>[2x]GAMESLPVIAAPSMWTRPQIKDFKEKIQQDADSVITVGRGEVVTVRVPTHEEGSYLFWEFATDNYDIGFGVYFEWTDSPNTAVSVHVSESSDDDEEEEENIGCEEKAKKNANKPLLDEIVPVYRRDCHEEVYAGSHQYPGRGVYLLKFDNSYSLWRSKSVYYRVYYTR;>[2x]GSGSGKPAPDAIGDLLASVDSEEVRQYCREQGWIIPETPTNVERHLNR

ACBD3 is a Golgi resident protein involved in the maintenance of the Golgi structure and regulation of intracellular trafficking between the endoplasmic reticulum and the Golgi. However, in enterovirus-infected cells, the ACBD3 GOLD domain interacts preferentially with viral non-structural 3A proteins, which causes re-localization of ACBD3 to the sites of virus replication. In this study, we present a structural, biochemical, and biological characterization of the complexes composed of human ACBD3 and the 3A proteins of four representative enteroviruses. The crystal structures revealed the details of the ACBD3-3A interaction, the 3A-3A interaction causing the assembly of the ACBD3-3A heterotetramers, the interaction between the ACBD3-3A complex and the lipid bilayer, and the roles of these interactions in facilitation of enterovirus replication.

The second strategy took advantage of the fact that in all three solved GOLD: 3A structures the C terminus of the ACBD3 GOLD domain was located in the vicinity of the N terminus of the ordered part of the 3A protein. This allowed us to design GOLD-3A fusion proteins with the last residue of ACBD3 (R528ACBD3) fused through a short peptide linker (GSGSG) to the first predicted ordered residues of the respective 3A proteins (e.g. K153A/EVA71). The overall structures of all solved GOLD: 3A complexes are highly similar to each other. This suggests that neither the L24A mutation in the GOLD: 3A/PV1 complex nor the fusion-protein strategy used for the GOLD: 3A/EVA71 complex affected the overall fold of the complexes. Analysis of the crystal structures of the GOLD: 3A complexes revealed that the 3A proteins formed either one of the crystal-packing contacts (as in the case of EVD68 and PV1) or contacts with the second 3A molecule when two GOLD: 3A complexes per asymmetric unit were present (as in the case of EVA71 and RVB14). This putative dimerization interface is formed by the two central alpha helices of the 3A proteins, which are bent 180° to form a helical hairpin. The dissociation constants of the GOLD: enterovirus 3A complexes ranged approximately from 1 μM (EVD68 and RVB14) to 15 μM (EVA71).>[6x]GPGSEFPDGTREFLTFE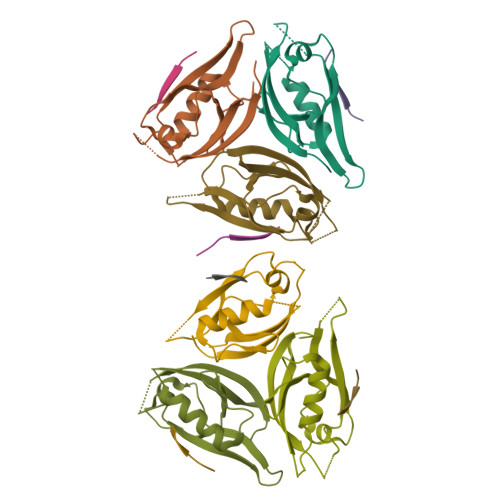VPLNDSGSAGLGVSVKGNRSKENHADLGIFVKSIINGGAASKDGRLRVNDQLIAVNGESLLGKANQEAMETLRRSMSTEGNKRGMIQLIVARRIS;>[6x]LCSNMEESFV2-(4-chlorophenyl)-~{N}-pyrimidin-2-yl-ethanamide | C12 H10 Cl N3 O | 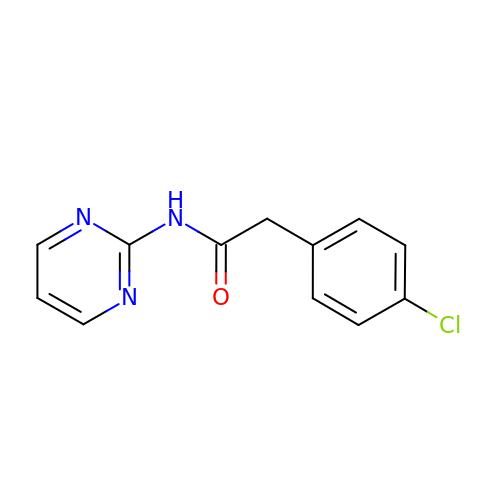RHMYHGQXWBKCMJ-UHFFFAOYSA-N>YFQSMRSPITIQRSGKKYGFTLRAIRVYMGDTDVYSVHHIVWHVEEGGPAQEAGLCAGDLITHVNGEPVHGMVHPEVVELILKSGNKVAVTTTPFENT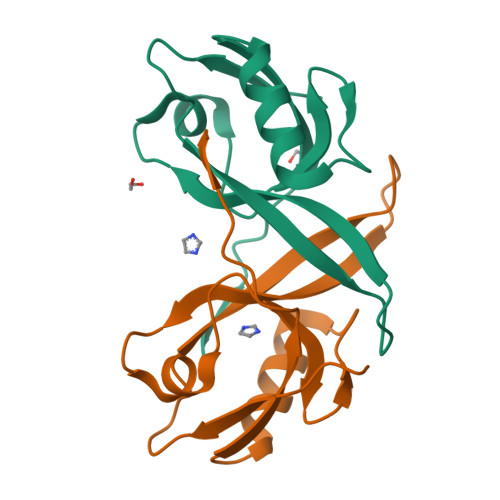QSLV[4x]Replication Protein A (RPA) is a heterotrimeric single stranded DNA-binding protein with essential roles in DNA replication, recombination and repair. In Archaea, the same function is also fulfilled by a heterotrimeric RPA. We report three crystal structures and five cryo-EM structures of Pyrococcus abyssi RPA (hereafter referred to PabRPA), in its apo form as well as bound to ssDNA. We find that archaeal and eukaryotic RPAs share a conserved heterotrimerization core, which is composed of three OB domains connected through a three-helix bundle formed by a C-terminal α-helix from each subunit.

Unexpectedly, aside from forming nucleoprotein filaments in the presence of ssDNA, we discovered that PabRPA oligomerizes in solution to form higher-order assemblies in the absence of ssDNA. At micromolar protein concentration range, PabRPA exists predominantly in the tetrameric form, as shown by SEC-SLS. The PabRPA tetrameric supercomplex is formed by two dimers (AB and CD) arranged in a C2-symmetrical assembly, which interact through contacts involving their Tri-Cs. Interactions within the AB and CD dimers involve their OB-3 domains, while the two dimers are held together by interactions involving their OB-4 domains. An interaction between AROD and OB-4 was also observed by Cryo-EM. By isolating a subset of the dataset through 3D classification, we determined an asymmetric 3.8 Å cryo-EM structure of the PabRPA tetrameric supercomplex showing the interaction between the OB-1 domain from one RPA complex and the OB-4 domain of another RPA. Instead, AROD participates in RPA-RPA inter-molecular protein-protein interactions.

>[4x]MSVLTKDRIIEIIERKTGMSREEIEEEIRKIMEEDPYLSEQGAAALLAERLGIDLIEKEEVSLMRISELYPGMDPREVNVVGRVLKKYPPREYTRKDGSVGRVASLIIYDDSGRARVVLWDAKVSEYYNKIEVGDVIKVLDAQVKESLSGLPELHINFRARIILNPDDPRVEMIPPLEEVRVATYTRKKIKDIEAGDRFVEVRGTIAKVYRVLTYDACPECKKKVDYDEGLGVWICPEHGEVQPIKMTILDFGLDDGTGYIRVTLFGDDAEELLGVSPEEIAEKIKELEESGLTTKEAARKLAEDEFYNIIGREIVVRGNVIEDRFLGLILRASSWEDVDYRREIERIKEELEKLGVM;>[4x]KKRMPATRLYIKDILEGYFVKSEGDFEPNYLITKYARKVYRAKIVGTVVREPLIAEDETYGKFQVDDGTGVIWVLGFRDDTKFAKLVRKGDLVQVIGKIAEWRDDKQILVEGVSKVHPNMWILHRYETLKEKIEHIKKAKIALEIYNQYGITAKSKVIAKNKGIEEELLEVIDELYGIMM;>[4x]RRRKPAVERKISEIREEDTRVSLIGRVIKVDKMDYMFWLDDGTGVAIIESESDLPKVGQVVRVIGRIIRNEEGIHIYAEVIQDFSDADLEALEEIRELERKLLPRLEGEIVW> MSDMEKPWKEEEKREVLAGHARRQAPQAVDKGPVTGDQRISVTVVLRRQRGDELEAHVERQAALAPHARVHLEREAFAASHGASLDDFAEIRKFAEAHGLTLDRAHVAAGTAVLSGPVDAVNQAFGVELRHFDHPDGSYRSYVGDVRVPASIAPLIEAVLGLDTRPVARPHFRLRRRAEGEFEARSQSAAPTAYTPLDVAQAYQFPEGLDGQGQCIAIIELGGGYDETSLAQYFASLGVSAPQVVSVSVDGATNQPTGDPNGPDGEVELDIEVAGALAPGAKIAVYFAPNTDAGFLNAITTAVHDPTHKPSIVSISWGGPEDSWAPASIAAMNRAFLDAAALGVTVLAAAGDSGSTDGEQDGLYHVDFPAASPYVLACGGTRLVASAG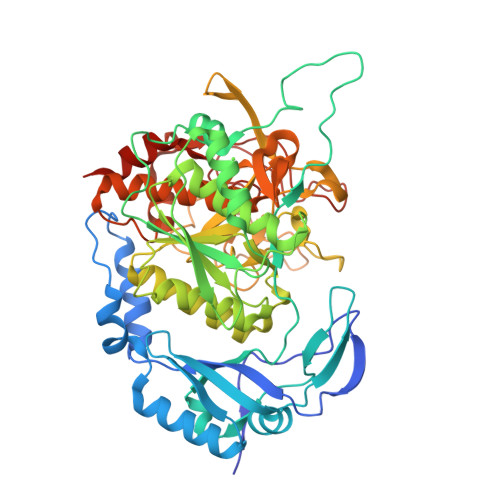RIERETVWNDGPDGGSTGGGVSRIFPLPSWQERANVPPSANPGAGSGRGVPDVAGNADPATGYEVVIDGETTVIGGTAAVAPLFAALVARINQKLGKPVGYLNPTLYQLPPEVFHDITEGNNDIANRARIYQAGPGWDPCTGLGSPIGIRLLQALLPSASQAQP>[2x]GKNGKGEVIIPKEKFWKISTPPEAYWNREQEKLNRQYNPILSMLTNQTGEAGRLSNISHLNYCEPDLRVTSVVTGFNNLPDRFKDFLLYLRCRNYSLLIDQPDKCAKKPFLLLAIKSLTPHFA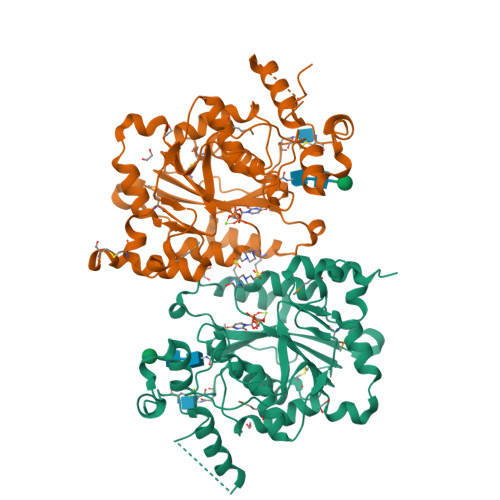RRQAIRESWGQESNAGNQTVVRVFLLGQTPPEDNHPDLSDMLKFESEKHQDILMWNYRDTFFNLSLKEVLFLRWVSTSCPDTEFVFKGDDDVFVNTHHILNYLNSLSKTKAKDLFIGDVIHNAGPHRDKKLKYYIPEVVYSGLYPPYAGGGGFLYSGHLALRLYHITDQVHLYPIDDVYTGMCLQKLGLVPEKHKGFRTFDIEEKNKNNICSYVDLMLVHSRKPQEMIDIWSQLQSAHLKC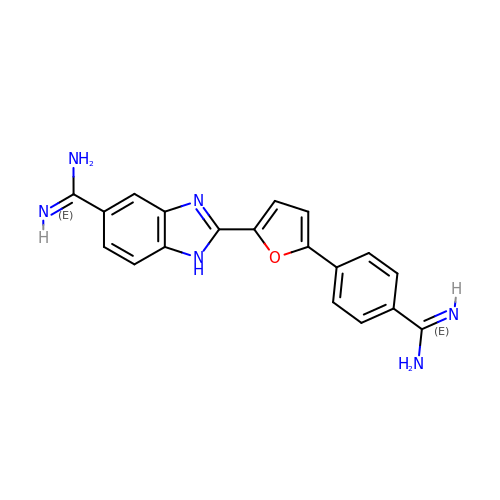2-(5-{4-[AMINO(IMINO)METHYL]PHENYL}-2-FURYL)-1H-BENZIMIDAZOLE-5-CARBOXIMIDAMIDE | C19 H16 N6 O | LXJNJISEUJIGFP-UHFFFAOYSA-N> GHMATVKKLYFVPAGRCMLDHSFVNSALTPGKLLNVPVWCYLLETEEGPILVDTGMPESAVNNEGLCNGTFGEGQILPKMTEEDRIVNILKRVGYEPDDLLYIISSHLHFDHAGGNGAFTNTPIIVQRTEYEAALHREEYMTECILPHLNYKIIEG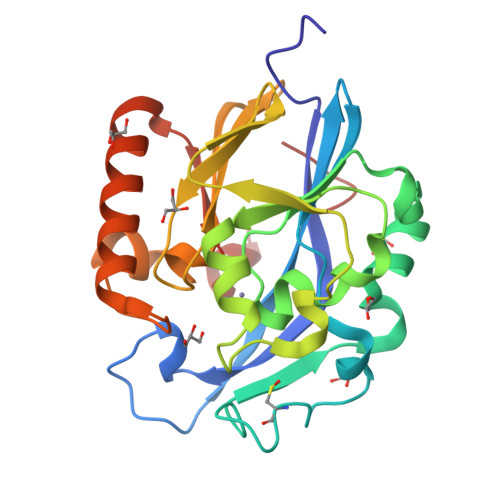DYEVVPGVQLLYTPGHSPGHQSLFIETEQSGSVLLTIDASYTKENFEDEVPFAGFDPELALSSIKRLKEVVKKEKPMIFFGHDIEQEKSCRVFPEYI>AESHWCYEVQAESSNYPCLVPVKWGGNCQKDRQSPINIVTTKAKVDKKLGRFFFSGYDKKQTWTVQNNGHSVMMLLENKASISGGGLPAPYQAKQLHLHWSDLPYKGSEHSLDGEHFAMEMHIVHEKEKGTSRNVKEAQDPEDEIAVLAFLVEAGTQVNEGFQPLVEALSNIPKPEMSTTMAESSLLDLLPKEEKLRHY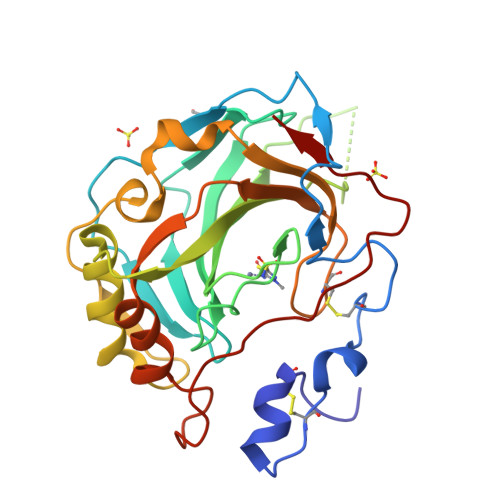FRYLGSLTTPTCDEKVVWTVFREPIQLHREQILAFSQKLYYDKEQTVSMKDNVRPLQQLGQRTVIKS[4x]>[2x]QRCGGWVKLNTAPVCFSAKGNRPGSFTPSHHGFLKSVKLRHLRGLVTCQSSTDAHDSYWG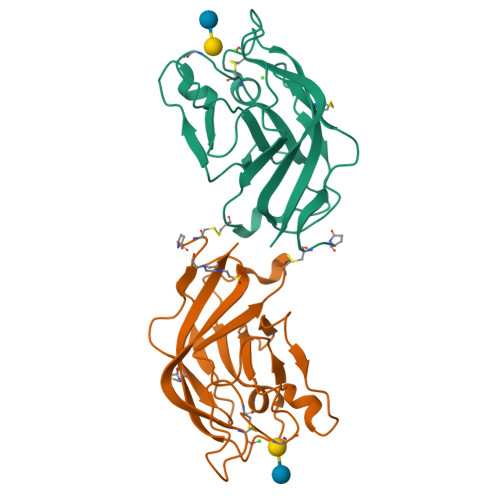CKNRNGFHNYPLNVFVTDKHNKVMFPKTGATYYLDPYVIKNRFYGVQGYNAMSPELVLQHGCNSPSDYIGPDSQLRVWYGEDLYNTMESDNSGKVCADVFGYFV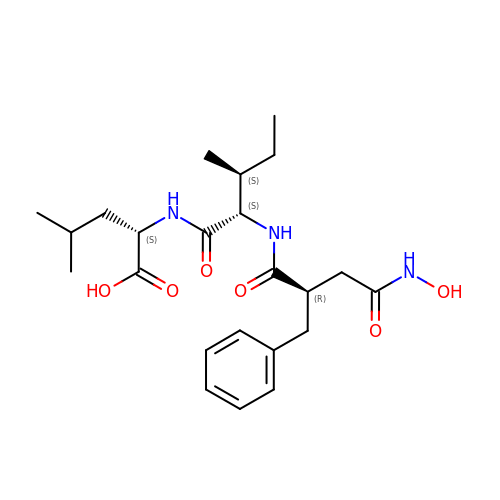N-[(2R)-2-BENZYL-4-(HYDROXYAMINO)-4-OXOBUTANOYL]-L-ISOLEUCYL-L-LEUCINE | C23 H35 N3 O6 | MWZOULASPWUGJJ-NFBUACBFSA-N> MEDKGKTFFGQPLGLSTLFMTEMWERFSYYGMRAILLYYMWFLISTGDLHITRATAASIMAIYASMVYLSG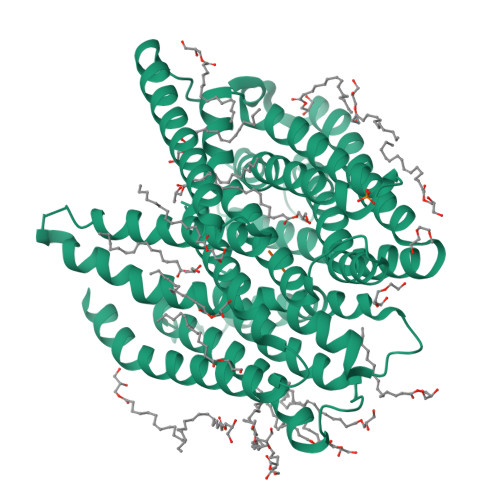TIGGFVADRIIGARPAVFWGGVLIMLGHIVLALPFGASALFGSIILIIIGTGFLKPNVSTLVGTLYDEHDRRRDAGFSIFVFGINLGAFIAPLIVGAAQEAAGYHVAFSLAAIGMFIGLLVYYFGGKKTLDPHYLRPTDPLAPEEVKPLLVKVSLAVAGFIAIIVVMNLVGWNSLPAYINLLTIVAIAIPVFYFAWMISSVKVTSTEHLRVVSYIPLFIAAVLFWAIEEQGSVVLATFAAERVDSSWFPVSWFQSLNPLFIMLYTPFFAWLWTAWKKNQPSSPTKFAVGLMFAGLSFLLMAIPGALYGTSGKVSPLWLVGSWALVILGEMLISPVGLSVTTKLAPKAFNSQMMSMWFLSSSVGSALNAQLVTLYNAKSEVAYFSYFGLGSVVLGIVLVFLSKRIQGL;> AF>ERMILIRGLTRVITFDDQERELEDADILIDGPKIVAVGKNLSDRSVSRTIDGRGMIALPGLINSHQHLYEGAMRAIPQLERVTMASWLEGVLTRSAGWWRDGKFGPDVIREVARAVLLESLLGGITTVADQHPFFPGATADSYIDATIEAATDLGIRFHAVRSSMTLGKSEGGFCDDLFVEPVDRVVQHCLGLIDQYHEPEPFGMVRIALGPCGVPHDKPELFEAFAQMAADYDVRLHTHFYQPLDAGMSDHLYGMTPWRFLEKHGWASDRVWLAHAVVPPREEIPEFADAGVAIAHLIAPDLRLGWGLAPIREYLDAGITVGFGTTGSASNDGGNLL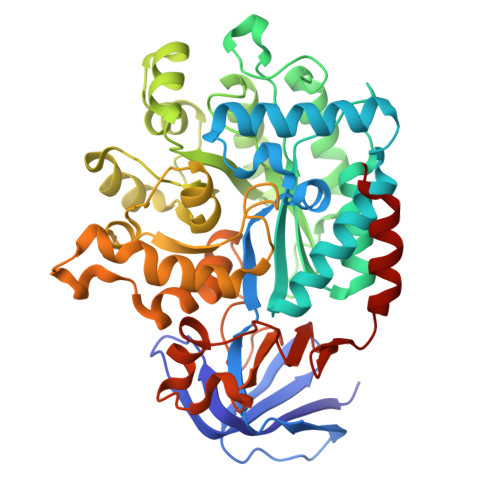GDLRLAALAHRPADPNEPEKWLSARELLRMATRGSAECLGRPDLGVLEEGRAADIACWRLDGVDRVGVHDPAIGLIMTGLSDRASLVVVNGQVLVENERPVLADLERIVANTTALIPKNL[2x]>GVSSDQVAVAGNAERLFNGAWYNLFEYGTTYANIGYRALQCQDDMMASDVVSRPKYGFNSSYQFNDVAIPSDGRTSFAWYLIYKTIDNCNTAISIKGDSEELRQAQGQALALRAFCYLHLVQHYQFTYLKDKDAPCVPIYTEPTTSGTKPKGKSTVAQVYQQIFDDLNLAQDYLTNYVRKGDGQKFKPNTDVVNGLMARAYLLTGQWGEAAKAAEAARKGYSLMTTTAEYEGFNNISNKEWIWGSPQTLSQSDASYNFYYLDATYVGAYSSFMADPHLMDTFVKGDIRLPLFQWMREGYLGYKKFHMRSDDTADLVLMRSAEMYLIEAEAKVRDGVALDQAVAPLNTLRTARGVGNYDVTGKTKEQVIDEILMERRRELWGEGFGITDVLRNQKAVERMALSEDMQKTEVDCWQEGGSFAKRNPLGHWFLNFP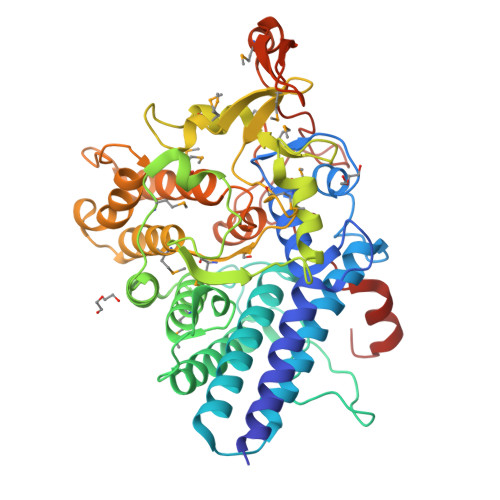DGKAFSANSSYYLYAIPEKEINANPNL[2x]2-acetamido-1-O-carbamoyl-2-deoxy-alpha-D-glucopyranose | C9 H16 N2 O7 | 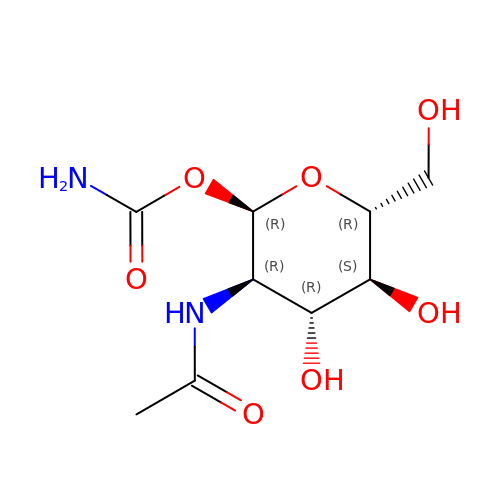BMFDLZBABRHLIB-FMDGEEDCSA-N> MNAIHIGPFSITPAARGLHYGGLPHHQWTLYYGPREMAIKTLPDSYTSSEVRDEFSDIIAEFVIDARHRYAPGSGSSGSAPPLAWITGLLPGEVLTHDAEEWRPPTSWELRHVV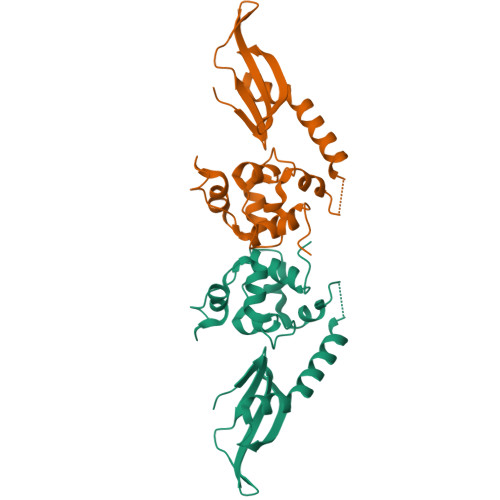GEGSFTGVSGAAAAALLGMSATNFRKYTAGDSAANRQKISFAAWHYLLDRLGVKRAS> TNTDSFTFSKFKPNQPNLKKQGDATVTSSGTLQLTKVDKNGVPDPKSLGRALYASPINIWDSKTGVVASFATSFRFTIYAPNIATIADGLAFFLAPVSSPPKAGAGFLGLF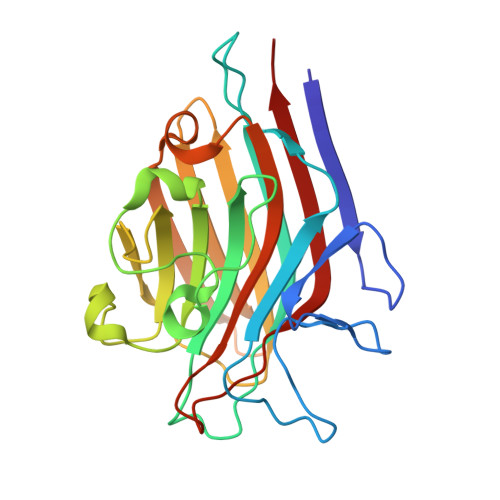DSAVFNSSYQTVAVEFDTYENTVFLDPPDTHIGIDVNSIKSIKTVKWDLANGEAAKVLITYDSSAKLLVAALVYPSSKTSFILSDVVDLKSVLPEWVSIGFSAATGASSGYIETHDVFSWSFASKLSF4-{2-[(6-amino-8-oxo-7,8-dihydro-1H-imidazo[4,5-g]quinazolin-2-yl)amino]ethyl}benzonitrile 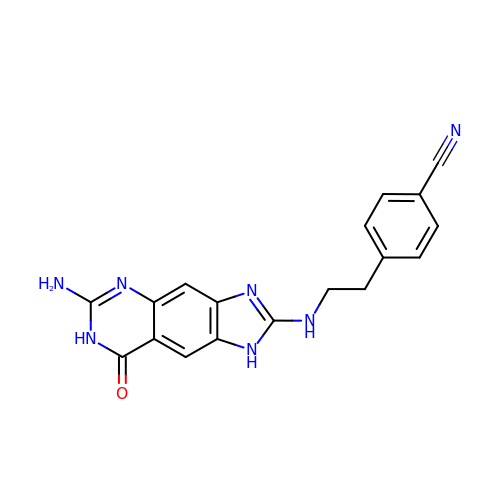| C18 H15 N7 O | NYFZULJQMISTPE-UHFFFAOYSA-N> MAEGNTLISVDYEIFGKVQGVFFRKHTQAEGKKLGLVGWVQNTDRGTVQGQLQGPISKVRHMQEWLETRGSPKSHIDKANFNNEKVILK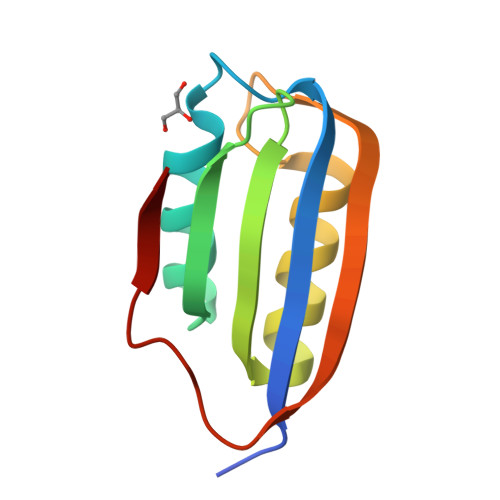LDYSDFQIVG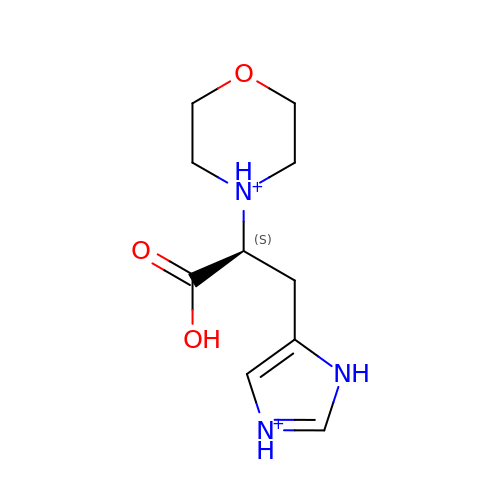Morpholinohistidine | C10 H17 N3 O3 | JPWIPIHZQZQXRJ-VIFPVBQESA-P> AIDEIKSRGYLLVGLSADFPPFEFVDENGNIVGFDVDLAKEIARRLGVELKIVDMTFDGLIPSLLTKKIDVIISGMTITEERKKVVAFSDPYFDAGQVIVVRKDSDFRPKTYEDLVGKTVAVQIGTTGDIEVSKYDGIKVVRFDKFTDAFLELKRGRADAVVLDSATARAFVAKNPDLVISSGVLSSEQYGIAVRKEDTDLLEFINSV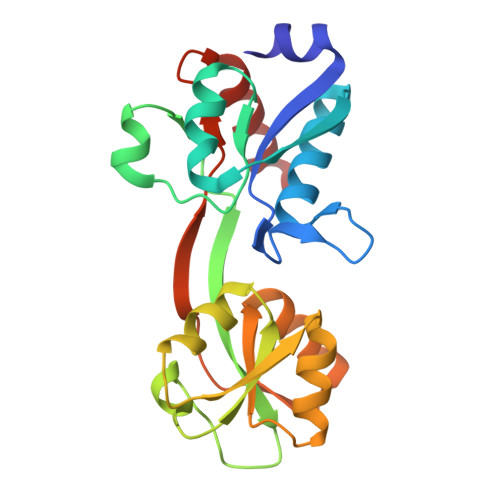LREL>[4x]GSHMSSPSDGPFPKATPQLPNSVFDMFSMKGKVTAITGGGGGIGFAAAEAIAEAGGDVALLYRSAPNMEERSAELAKRFGVKVKSYQCEVTEHESVKQAIEAVEKDFGRLDCYIANAGGGVPGSINPDYPLEAWHKTQSVNLHSTFYAARECA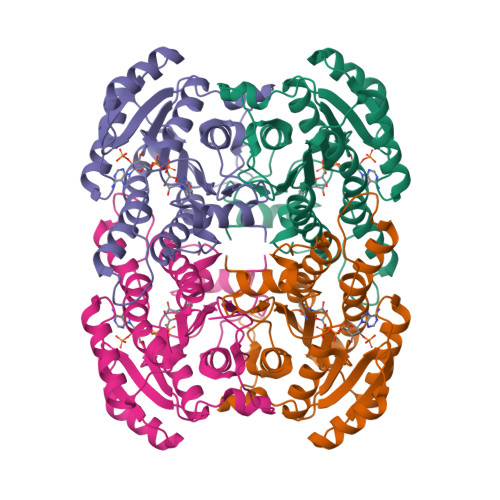RIFKAQGSGSFIATTSISARIVNVPYDQPAYNSSKAAVVHFCRSLARDWRNFARVNTISPGFFDTPMGPSDKAVEDVLYQKSVLGRAGDVKELKAAYLYLASNASTYTTGADLLIDGGYCLT>GSHMATGKEYEVIKNDVEHDMKADHITYEGLNKEATEGYRITANQKSFSKEEIEALKDQKPLMDMPSDDHKVTSLKMKFANPIALSKKDIEDDAQALVSSKIQDGEKYKLWKVDKSKKEIIFFQTYEGHYIYQKTDNPSNMIGQVVLHLNGKNEVVSYDQTTLETFKQIQKESLITEMDAVELLYYQNQLKE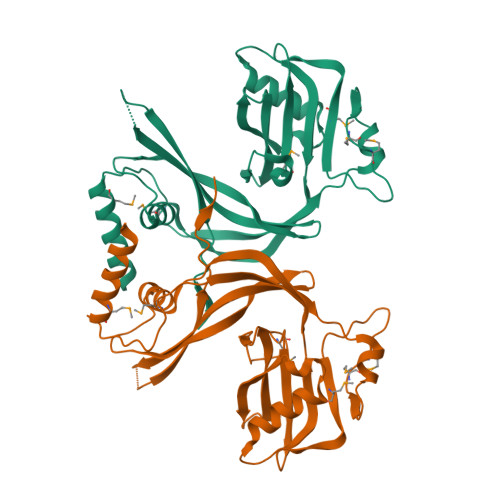YSTVKSCKFGYVAQYPLTSTQVLAPVWRITVEYEKKVNGEKKTVQEYFTVNALESTILDTDQ[12x]>[2x]MVRPSQSMYDRHLTIFSPDGNLYQIEYAIKAVKNTNITSVGVKGENCAVIISQKKMATQYISQDKLLDYNNITNIYNITDEIGCSMVGMPGDCLSMVYKARSEASEFLYSNGYNVNAETLCRNICDKIQVYTQHAYMRLHACSGMIIGIDENNKPELFKFDPSGFCAGYRACVIGNKEQESISVLERLLEKRKKKIQQETIDEDIRNTTILAIEALQTILAFDLKASEIEVAIVSTKNRNFTQISEKEIDNYLTYIAERD;>MADGEYSFSLTTFSPTGKLVQIEYALNRVSSSSPALGIRAKNGVIIATEKKSPNELIEENSIFKIQQISEHIGIVYAGMPGDFRVLLKRARKEAIRYSLQYGSEILVKELVKIIASIVQEFTQTGGVRPFGLSLLICGVDVYGYHLYQIDPSGCYFNWMATCVGKDYQNNMSFLEKRYNKDIEIEDAIHTAILTLKESYEGVLNEKNIEIGVAYDNKPFKILTQNEIKDYLIEIE[2x];>[2x]MARRYDSRTTTFSPEGRLYQVEYALEAINNASITIGLITKDGVILGADKVFISKLIDKANNYEKIYKIDKHIFCGVAGLNADANILINQSRLYAQRYLYNYNEVQPVSQLVVQICDIKQSYTQYGGLRPYGVSFLIGGYDTKDGYQLYHTDPSGNYSGWFATAIGTNNLTASSVLKQEWKNDMTLEEGLLLALKTLAKSTDTEIPKSEKIELAYLTNKDGEVYQKYLTEKEIEELIKLYTQK;>MSYDRAITVFSPDGHLLQVEHALEAVKKGGCAVAIKSSNFAVLAVEKKNIPKLQNPKTTEKLIKLDEHNCLAFAGLNADARVLVNKTRLECQRYYLNMDEPAPVDYIAKYVAKVQQKFTHRGGVRPFGIATLIAGFKNNKEICIYQTEPSGIYAAWKAQAIGKNAKIVQEFLEKNYQENMEQKDCIFLALKAIFEVVELSSKNVEVALLTEKDLTFIEEQEINSMVELIDQERTKNNEQNE[2x];>[2x]MFSTRSEYDRGVNTFSPEGRLFQVEYALGAIKLGSTAVGICVNDGVILASERRISSTLIEKDSVEKLLSIDDHIGCAMSGLMADARTLIDYARVECNHYKFIYNENINIKSCVELISELALDFSNLSDSKRKKIMSRPFGVALLIGGVDKNGPCLWYTEPSGTNTRFSAASIGSAQEGAELLLQENYKKDMTFEQAEILALTVLRQVMEDKLSTSNVEICAIKKSDQTFYKYNTDDISRIIDVLPSPVYPTIDMTA;>MYRNLYDTDNIIYSPEGRLYQVEYASEAIKQGTCAVAIKSKDYVVVSGLKKCISKLSFPQEKIFKIDDYIGISMSGITSDAKVLTKFMQNECLSHKFLYNENINIESLVRSVADKYQKNTQKSSKRAFGVGLMIAAYHNEPCIFETRPNGSYFEYDALSFGARSHASKTYLEKNLHLFEECSLEELILHCLKALKCSLSSESELTISNTALAVVGKNHPWQEISSLQLEEYLSKVKMDAEQEQVEENVQNEANE[2x];>[2x]MAGLSAGYDLSVSTFSPDGRLYQVEYIYKSINNNNTALCLECKDGIICCCINSNMDKNKMIKKNSYNRIYHVNNNIIITYSGFDGDARNIIDRARSEANTYYYNFHTNIPLHILVNRISLYIHAYTLYWHMRPFAASIIISSFNEKDKGDIYCIEPNGACYKYSGIVIGKNKEMFK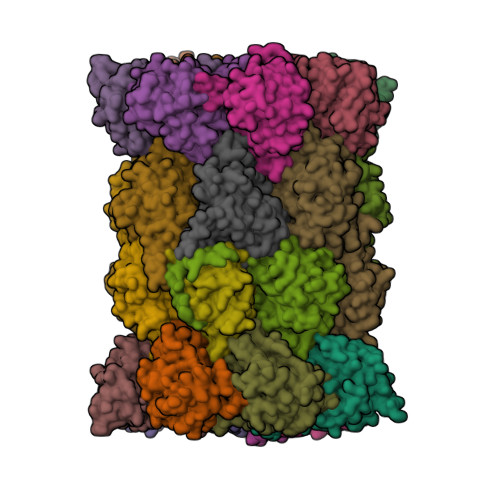TEIEKKDYKDINVRDAIEDIYKFILTSDDHMNKNNLQNLVNFSWICKESSYEFQNIHEEILTPALNKAVEYIEKLN;>[2x]TTIIGIIYDNGVMLACDSRTSSGTFISNKCSRKINRINENLYVCRSGASAHSQKIIEIIKHYCVSMKNENRKKGRFHEGETIYDETTYDEEIDIDSINYLDYNNNNDNNLVTKNKYFYEDKFNDYNPLVENVAHITKKIIYTNNNFLSCALIFGGYDKIKKQQLYAVNLNGSIIEKHDFAVSGSGSIYIQSYLQDKYKKFMTKKECFNLILNCVKYAMHNDNSSGGLIRIVNITKSFVEEFTVVNTQMNFQY;>TTICGLVCQNAVILGADTRATEGPIVADKNCSKLHYISKNIWCAGAGVAGDLEHTTLWLQHNVELHRLNTNTQPRVSMCVSRLTQELFKYQGYKVCAIVLGGVDVNGPQLYGIHPHGSSCLLPFTALGSGSLNAMAVLEAKYRDNMTIEEGKNLVCEAICAGIFNDLGSGGNVDICVITKDSYQHIRPYKEPNMRLYHLPHPTIYPKGTTPILSEKIEYIKKFISVEDA[2x];>MGSIYNYNGGCVLGMSGSNCVAIACDLRLGANTFTTVSTKFSKIFKMNNNVYVGLSGLATDIQTLYEILRYRVNLYEVRQDAEMDVECFANMLSSILYSNRFSPYFVNPIVVGFKLKHYVDEEGEKKVNYEPYLTAYDLIGAKCETRDFVVNGVTSEQLFGMCESLYVKDQDENGLFETISQCLLSALDRDCISGWGAEVLVLTPEKIIKKKLKARMD[2x];>[2x]MDTLIGLRGNNFVVLAADTYSINSIIKLKNDDNTKFYDIHGNKCLLLGGSIGDRLQFGEFIRKNVHLYQYQNNTDMFVKSFAFFTRKNLAYYLRRNPFEVNCLIAGYDKKDGYQLYWCDYLSNMDSVNKGAHGYGAYLVSAILDKYYHENLTVDEALDIFKLCFEELKKRFLLTQINYELRIMYDNKVETQYVTV;>[2x]TTTLAFKFKDGIIVAVDSRASMGSFISSQNVEKIIEINKNILGTMAGGAADCLYWEKYLGKIIKIYELRNNEKISVRAASTILSNILYQYKGYGLCCGIILSGYDHTGFNMFYVDDSGKKVEGNLFSCGSGSTYAYSILDSAYDYNLNLDQAVELARNAIYHATFRDGGSGGKVRVFHIHKNGYDKIIEGEDVFDLHYHYTNPEQKDQYVM;>MDLILYNDNLTEKKTEKENVIEHGRGFKRWYPYIDNGGTVIGLTGKDYVILAADTRLSLSYSIYTRFCPKISKLTDKCIIGSSGMQSDIKTLHSLLQKKIQLFVLEHSHYPDIHVIARLLCVILYSRRFFPYYAFNILAGVDENNKGVLYNYDSVGSYCEATHSCVGSGSQLILPILDNRVEQKNQLIKNTNFNLGDDINFVKDAITSATERDIYTGDKTLIYVIDKMGINVNTLDLKQD[2x];>[2x]MTLGPVVTGTSVIAIKYKHGIMIAADRKASYGSYAKFQNVERIFKINNKTVMGFSGELADAQYLHELLTRKNINNLSEKKRKEDMYTPQHYHSYVSRVFYVRKNRIDPLFNNIIIAGINSQKYDNNDDNVLLYTNKNNDDEQNEYKNNEEYKEIHKDDLYIGFVDMHGTNFCDDYITTGYARYFALTLLRDHYKDNMTEEEARILINECLRILYFRDATSSNFIQIVKVTSKGVEYEEPYILPCVLNSADYVYPSTLLPPAGCMWGSGSENLYFQGHHHHHHHH> MRRETVGEFSSDDDDDILLELGTRPPRFTQIPPSSAALQTQIPTTLEVTTTTLNNKQSKNDNQLVNQLNKAQGEASMLRDKINFLNIEREKEKNIQAVKVNELQVKHLQELAKLKQELQKLEDEKKFLQMEARGKSKREVITNVKPPSTTLSTNTNTITPDSSSVAIEAKPQSPQSKKRKISDNLLKKNMVPLNPNRIIPDETSLFLESILLHQIIGADLSTIEILNRLKLDYITEFKFKNFVIAKGAPIGKSIVSLLLRCKKTLTLDRFIDTLLEDIAVLIKEISVHPNESKLAVPFLVALMYQIVQFRPSATHNLALKDCFLFICDLIRIYHHVLKVPIHESNMNLHVEPQIFQYELIDYLIISYSFDLLEGILRVLQSHPKQTYMEFFDENILKSFEFVYKLALTISYKPMVNVIFSAVEVVNIITSIILNMDNSS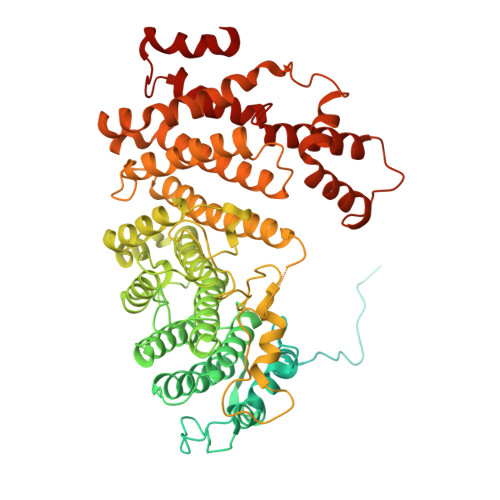DLKSLISGSWWRDCITRLYALLEKEIKSGDVYNENVDTTTLHMSKYHDFFGLIRNIGDNELGGLISKLIYTDRLQSVPRVISKEDIGMDSDKFTAPIIGYKMEKWLLKLKDEVLNIFENLLMIYGDDATIVNGEMLIHSSKFLSREQALMIERYVGQDSPNLDLRCHLIEHTLTIIYRLWKDHFKQLREEQIKQVESQLIMSLWRFLVCQTETVTANEREMRDHRHLVDSLHDLTIKDQASYYEDAFEDLPEYIEEELKMQLNKRTGRIMQVKYDEKFQEMARTILESKSFDLTTLEEADSLYISMGL>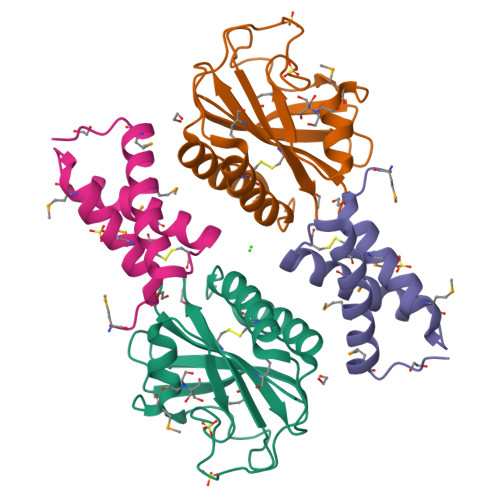 MNVDPHFDKFMESGIRHVYMLFENKSVESSEQFYSFMRTTYKNDPCSSDFECIERGAEMAQSYARIMNIKLETE;> RFESVALEQLQIVHISSEADFSAVYSFRPKNLNYFVDIIAYEGKLPSTISEKSLGGYPVDKTMDEYTVHLNGRHYYSNSKFAFLPTKKPTPEINYMYSCPYFNLDNIYAGTITMYWYRNDHISNDRLESICAQAARILGRAKKLAAALEHHHHHH> MVGNPMWERDKIIVLGHRGYMAKYPENSLLSIRKAIEAGADGVEIDVWLSKDNKVILMHAETIDRTSNLKGRQKEMTLEELKKANIGMGERIPTLEEV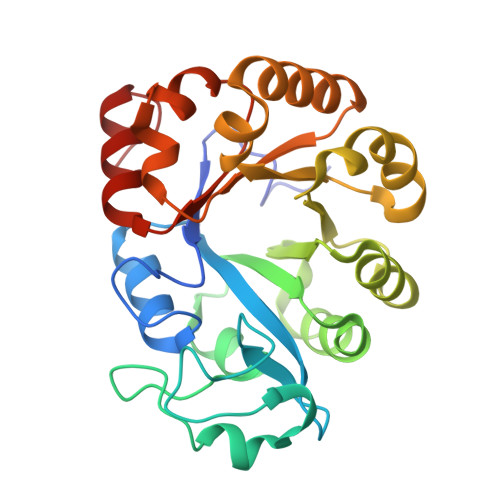FEILPKDALLNIEIKDRDAAKEVARIVSENNPERVMISSFDIEALREYRKYDDTTIMGLLVDKEETVPLIPKLKEKLNLWSVNVPMEAIPIIGFEKTYQAIKWVRSLGLKIVLWTEDDKLFYVDENLKRLLGMFEVVIANDVERMVSYLSSLGIRLE> VAQGPNGRALAESMNPDLLSAIQQHISIERYASV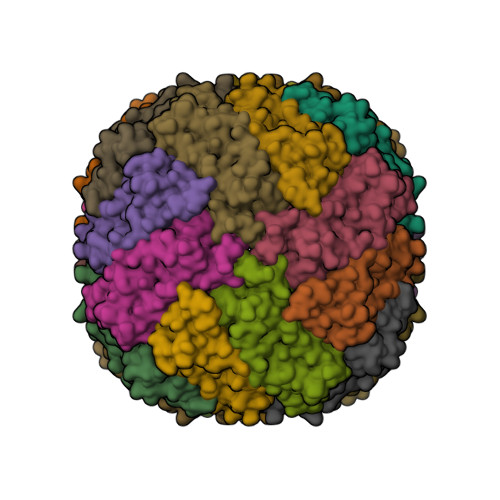TYLAMSIWCAERELAGFYQFFDGEAKDEQSHAVHFTQYLIARSQSNDLQTLDAPRQNWDSLASLMATAFQMEADTTSSIQSVYALAERNSDTRTTVFLDPLIEAQIQSEDQFAYLLGRVKFANGDPTALLVIDNELRAGQTQR>SNASKMSDVKCTSVVLLSVLQQLRVESSSKLWAQCVQLHNDILLAKDTTEAFEKMVSLLSVLLSMQGAVDINKLCEEMLDNRATLQ[2x];>EDKRAKVTSAMQTMLFTMLRKLDNDALNNIINNARDGCVPLNIIPLTT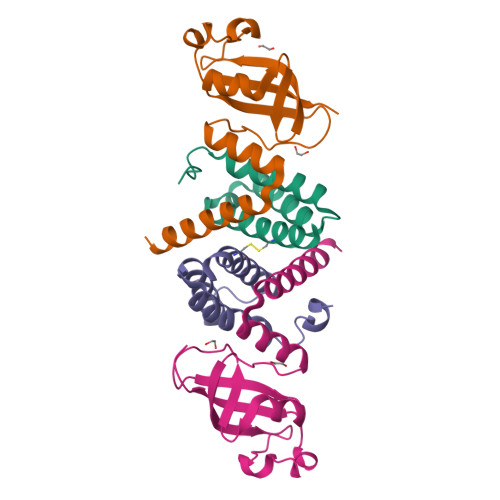AAKLMVVIPDYNTYKNTCDGTTFTYASALWEIQQVVDADSKIVQLSEISMDNSPNLAWPLIVTALRANSAVKLQ[2x]> MHHHHHHLVPRGSEDELYRQSLEIISRYLREQATGAKDTKPMGRSGATSRKALETLRRVGDGVQRNHETAFQGMLRKLDIKNEDDVKSLSRVMIHVFSDGVTNWGRIVTLISFGAFVAKHLKTINQESCIEPLAESIT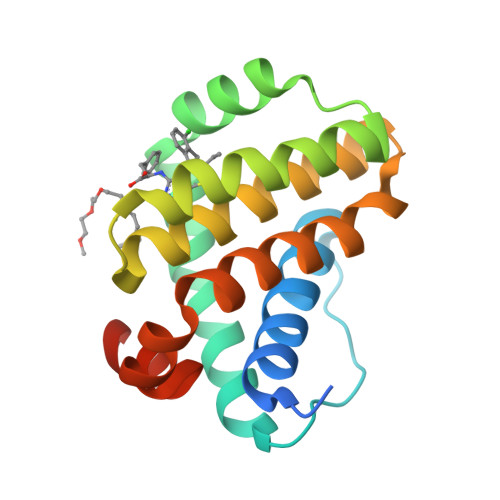DVLVRTKRDWLVKQRGWDGFVEFFHVEDLEGG> VDLLAVK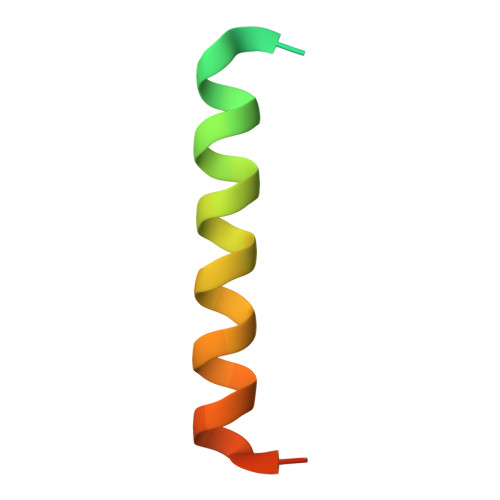KKQETKRSINEEIHTQFLDHLLTGIEDICGHYGHHH> MNYNLSKYPDDVSRLFKPRPPLSYKRPTDYPYAKRQTNPNITGVANLLSTSLKHYMEEFPEGSPNNHLQRYEDIKLSKIKNAQLLDRRLQNWNPNVDPHIKDTDPYRTIFIGRLPYDLDEIELQKYFVKFGEIEKIRIVKDKITQKSKGYAFIVFKDPISSKMAFKEIGVHRGIQIKDRICIVDIERGRTVKYFKPRRLGGGLGGRGYSNRDSRLPGRFASASTSNPAERNYAPRLPRRETSSSAYSADRYGSSTLDARYRGNRPLLSAATPTAAVTSVYKSRNSRTRESQPAPKEAPDY;> MTRYYCEYCHSYLTHDTLSVRKSHLVGKNHLRITADYYRNKARDIINKHNHKRRHIGKRGRKERENSSQNETLKVTCLSNKEKRHIMHVKKMNQKELAQTSIDTLKLLYDGSPGYSKVFVDANRFDIGDLVKASKLPQRANEKSAHHSFKQTSRSRDETCESNPFPRLNNPKKLEPPKILSQWSNTIPKTSIFYSVDILQTTIKESKKRMHSDGIRKPSSANGYKRRRYGN;> MSALYFQNLPSRPANKENYTRLLLKHINPNNKYAINPSLPLPHNKLQISSQPLMLLDDQMGLLEVSISRSSKMTNQAFLTFVTQEEADRFLEKYTTTALKVQGRKVRMGKARTNSLLGLSIEMQKKKGNDETYNLDIKKVLKARKLKRKLRSDDICAKKFRLKRQIRRLKHKLRSRKVEEAEIDRIVKEFETRRLENMKSQQENLKQSQKPLKRAKVSNTMENPPNKVLLIQNLPSGTTEQLLSQILGNEALVEIRLVSVRNLAFVEYETVADATKIKNQLGSTYKLQNNDVTIGFAK;> MDKYTALIHDENFSTLTLNVSRYPKSLAYWEKLLNYIVKASAPICKSTEPQLLKLIRCTYSSMLNEFPYLENYYIDFALLEYKLGNVSMSHKIFQRGLQAFNQRSLLLWTSYLKFCNNVISHQKQLFKKYETAEEYVGLHFFSGEFWDLYLEQISSRCTSSKKYWNVLRKILEIPLHSFSKFYALWLQRIDDIMDLKQLSQLTSKDELLKKLKIDINYSGRKGPYLQDAKKKLKKITKEMYMVVQYQVLEIYSIFESKIYINYYTSPETLVSSDEIETWIKYLDYTITLQTDSLTHLNFQRALLPLAHYDLVWIKYSKWLINSKNDLLGAKNVLLMGLKFSLKKTEIIKLLYSVICKLNEYVLLRNLLEKIESSYSDNVENVDDFEIFWDYLQFKTFCQNSLYSSRYSDSQSNGLLNKELFDKVWKRLSCKEKKSGQEILLNNLVQFYSKDTVEFVEKNIFQKIIEFGWEYYLQNGMFWNCYCRLIYFDTSRSYLDKRQYIVRKIWPQIDKKFAQSVLPSLTEFCESYFPEEMDTLEEMFTEEP;> MPDETNFTIEDIEPRPDALRGLDTQFLQDNTALVQAYRGLDWSDISSLTQMVDVIEQTVVKYGNPNDSIKLALETILWQILRKYPLLFGFWKRFATIEYQLFGLKKSIAVLATSVKWFPTSLELWCDYLNVLCVNNPNETDFIRNNFEIAKDLIGKQFLSHPFWDKFIEFEVGQKNWHNVQRIYEYIIEVPLHQYARFFTSYKKFLNEKNLKTTRNIDIVLRKTQTTVNEIWQFESKIKQPFFNLGQVLNDDLENWSRYLKFVTDPSKSLDKEFVMSVFDRCLIPCLYHENTWMMYIKWLTKKNISDEVVVDIYQKANTFLPLDFKTLRYDFLRFLKRKYRSNNTLFNNIFNETVSRYLKIWPNDILLMTEYLCMLKRHSFKNSLDQSPKEILEKQTSFTKILETSITNYINNQIDAKVHLQTLINDKNLSIVVVELIKTTWLVLKNNMQTRKYFNLYQKNILIKNSVPFWLTYYKFEKSNVNFTKLNKFIRELGVEIYLPTTVMNDILTDYKTFYLTHSNIVTYESSIIDSNTFDPILYPELKMSNPKYDPVLNTTANVDWHKKTEWKEAGHIGITTERPQISNSIIECNSGTLIQKPISLPNFRNLEKINQVKINDLYTEEFLKEGK;> MSYKQTTYYPSRGNLVRNDSSPYTNTISSETNNSSTSVLSLQGASNVSLGTTGNQLYMGDLDPTWDKNTVRQIWASLGEANINVRMMWNNTLNNGSRSSMGPKNNQGYCFVDFPSSTHAANALLKNGMLIPNFPNKKLKLNWATSSYSNSNNSLNNVKSGNNCSIFVGDLAPNVTESQLFELFINRYASTSHAKIVHDQVTGMSKGYGFVKFTNSDEQQLALSEMQGVFLNGRAIKVGPTSGQQQHVSGNNDYNRSSSSLNNENVDSRFLSKGQSFLSNGNNNMGFKRNHMSQFIYPVQQQPSLNHFTDPNNTTVFIGGLSSLVTEDELRAYFQPFGTIVYVKIPVGKCCGFVQYVDRLSAEAAIAGMQGFPIANSRVRLSWGRSAKQTALLQQAMLSNSLQVQQQQPGLQQPNYGYIPSSTCEAPVLPDNNVSSTMLPGCQILNYSNPYANANGLGSNNFSFYSNNNATNTQATSLLADTSSMDLSGTGGQQVIMQGSEAVVNSTNAMLNRLEQGSNGFMFA;> MRPRRRGLAYHHTKPKGQLSQGHYPTTSNDGQRRKVGNSEAFQSFDIWKNLDRIRSTKKNAGQFIKGSLLILPMRTEDKQQFDECMDELHKYISKDILRCYPQKEQKDEGMLFYIVLKDFNILDSCFVLSVLLAFQKRLWMAPSEKSYFRVPKNINLTGSFYLPKNIETGRGHIITSYRREQPSSSIVEVGFNVVPDFQQFQVKACHVSKFMNELSNFFSQVEFGKCEANVINYFKREYNRTYSQISLALYELPLIGDGLFDIKSYISKTRPIIETSKAQMIKHISEMKAYNEISGLQGDQFPRQQRPLSNSPSSNSISSSQTIEAGATSYQTQPQRHAVNKPSNVLNSSNRHSGPKTFEDGRYSEGNKPGFMTQDEIKQHCIGTIKASMDAVKKKSSYQILKTYVRCPRQNYIDIVYQNLNDLRSKTNCNIVVLNLNNLHESQMWLESLNTTNYTIFAQAPHPSTIRVISIGGVGEYIVKALELILNILEH;> MRDIVFVSPQLYLSSQEGWKSDSAKSGFIPILKNDLQRFQDSLKHIVDARNSLSETLLNSNDDGSIHNSDQNTGLNKDKEASIADNNSANKCATSSSRYQELKQFLPISLDQQIHTVSLQGVSSSFSRGQIESLLDHCLNLALTETQSNSALKVEAWSSFSSFLDTQDIFIRFSKVDEDEAFVNTLNYCKALFAFIRKLHEDFKIELHLDLNTKEYVEDRTGTIPSVKPEKASEFYSVFKNIEDQTDERNSKKEQLDDSSTQYKVDTNTLSDLPSDALDQLCKDIIEFRTKVVSIEKEKKMKSTYEESRRQRHQMQKVFDQIRKNHSGAKGSANTEEEDTNMEDEDEEDDTEDDLALEKRKEERDLEESNRRYEDMLHQLHSNTEPKIKSIRADIMSAENYEEHLEKNRSLYLKELLHLANDVHYDHHRSFKEQEERRDEEDRAKNGNAKELAPIQLSDGKAISAGKAAAITLPEGTVKSENYNADKNVSESSEHVKIKFDFKKAIDHSVESSSEDEGYRESELPPTKPSERSAAEDRLPFTADELNIRLTNLKESRYVDELVREFLGVYEDELVEYILENIRVNQSKQALLNELRETFDEDGETIADRLWSRKEFRLG;> MSTMSTPAAEQRKLVEQLMGRDFSFRHNRYSHQKRDLGLHDPKICKSYLVGECPYDLFQGTKQSLGKCPQMHLTKHKIQYEREVKQGKTFPEFEREYLAILSRFVNECNGQISVALQNLKHTAEERMKIQQVTEELDVLDVRIGLMGQEIDSLIRADEVSMGMLQSVKLQELISKRKEVAKRVRNITENVGQSAQQKLQVCEVCGAYLSRLDTDRRLADHFLGKIHLGYVKMREDYDRLMKNNRTTNASKTATTLPGRRFV;> MSKIQVAHSSRLANLIDYKLRVLTQDGRVYIGQLMAFDKHMNLVLNECIEERVPKTQLDKLRPRKDSKDGTTLNIKVEKRVLGLTILRGEQILSTVVEDKPLLSKKERLVRDKKEKKQAQKQTKLRKEKEKKPGKIAKPNTANAKHTSSNSREIAQPSSSRYNGGNDNIGANRSRFNNEAPPQTRKFQPPPGFKRK;> MKLVNFLKKLRNEQVTIELKNGTTVWGTLQSVSPQMNAILTDVKLTLPQPRLNKLNSNGIAMASLYLTGGQQPTASDNIASLQYINIRGNTIRQIILPDSLNLDSLLVDQKQLNSLRRSGQIANDPSKKRRRDFGAPANKRPRRGL;> MSSQIIDRPKHELSRAELEELEEFEFKHGPMSLINDAMVTRTPVIISLRNNHKIIARVKAFDRHCNMVLENVKELWTEKKGKNVINRERFISKLFLRGDSVIVVLKTPVE;> MTMNGIPVKLLNEAQGHIVSLELTTGATYRGKLVESEDSMNVQLRDVIATEPQGAVTHMDQIFVRGSQIKFIVVPDLLKNAPLFKKNSSRPMPPIRGPKRR;> MSNKVKTKAMVPPINCIFNFLQQQTPVTIWLFEQIGIRIKGKIVGFDEFMNVVIDEAVEIPVNSADGKEDVEKGTPLGKILLKGDNITLITSAD;> MSESSDISAMQPVNPKPFLKGLVNHRVGVKLKFNSTEYRGTLVSTDNYFNLQLNEAEEFVAGVSHGTLGEIFIRCNNVLYIRELPN;> MVSTPELKKYMDKKILLNINGSRKVAGILRGYDIFLNVVLDDAMEINGEDPANNHQLGLQTVIRGNSIISLEALDAI;> AAAAAAAAAAAAAAAAAAAAAAAAAAAAAAAAAAAAAAAAAAAAAAAAA;> MARPIDVSQLIAGINKKKGLDENTSGKISKPRFLNKQERSKQERLKENE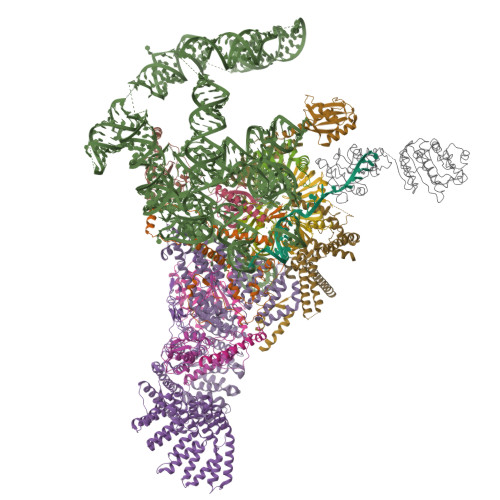ESLTPTQSDSAKVEIKKVNSRDDSFFNETNDKKRNPSKQNGSKFHFSWNESEDTLSGYDPIVSTRAIDLLWKGKTPKNAAESSYMGKHWTEKSLHEMNERDWRILKEDYAIVTKGGTVENPLRNWEELNIIPRDLLRVIIQELRFPSPTPIQRITIPNVCNMKQYRDFLGVASTGSGKTLAFVIPILIKMSRSPPRPPSLKIIDGPKALILAPTRELVQQIQKETQKVTKIWSKESNYDCKVISIVGGHSLEEISFSLSEGCDILVATPGRLIDSLENHLLVMKQVETLVLDEADKMIDLGFEDQVTNILTKVDINADSAVNRQTLMFTATMTPVIEKIAAGYMQKPVYATIGVETGSEPLIQQVVEYADNDEDKFKKLKPIVAKYDPPIIIFINYKQTADWLAEKFQKETNMKVTILHGSKSQEQREHSLQLFRTNKVQIMIATNVAARGLDIPNVSLVVNFQISKKMDDYIHRIGRTGRAANEGTAVSFVSAAEDESLIRELYKYVRKHDPLNSNIFSEAVKNKYNVGKQLSNEIIY> KFSKEQLRTFQMIHENFGRALSTYLSGRLRTFVDVEISIDQLTYEEFIRSVMIPSFIVIFTGDVFEG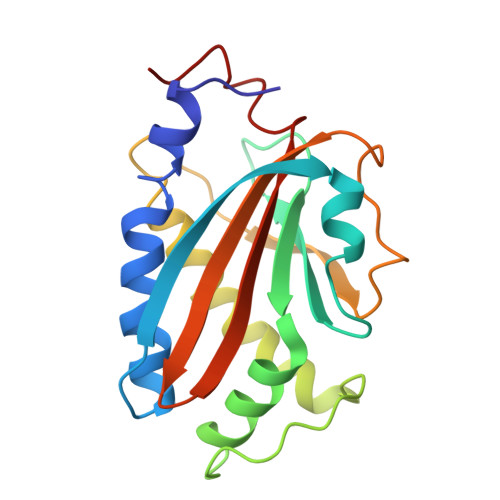SAIFEMRLDLFYTMLDIIMGGPGENPPNRPPTEIETSIMRKEVTNMLTLLAQAWSDFQYFIPSIENVETNPQFVQIVPPNEIVLLVTASVSWGEFTSFINVCWPFSLLEPLLEKLS> X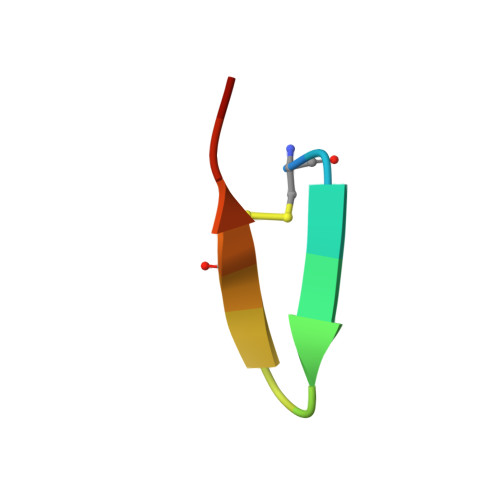CRAWYQNYCALRRX> MKDDQRWQSVLARDPNADGEFVFAVRTTGIFCRPSCRARHALRENVSFYANASEALAAGFRPCKRCQPDKAN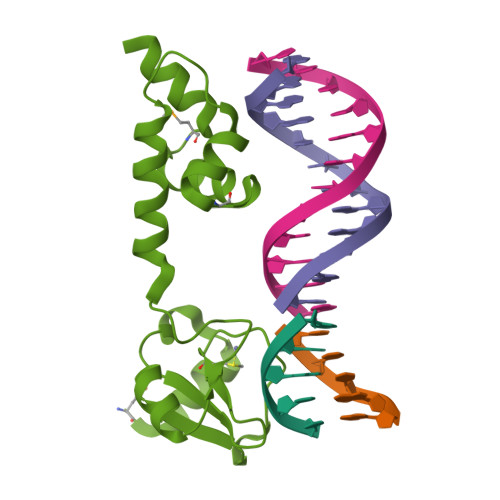PRQHRLDKITHACRLLEQETPVTLEALADQVAMSPFHLHRLFKATTGMTPKAWQQAWRARR>AFEDRDPTQFEERHLKFLRQLGKGNFGSVEMCRYDPLQDNTGEVVAVKKLQHSTEEHLRDFEREIEILKSLQHDNIVKYKGVCYSAGRRNLKLIMEFLPYGSLREYLQKHKERIDHIKLLQYTSQICKGMEYLGTKRYIHRDLATRNILVENENRVKIGDFGLTKVLPQDKEYYKVKEPGESPIFWYAPESLTESKFSVASDVWSFGVVLYELFTYIEKSKSPPAEFMRMIGNDKQGQMIVFHLIELLKNNGRLPRPDGCPDEIYMIM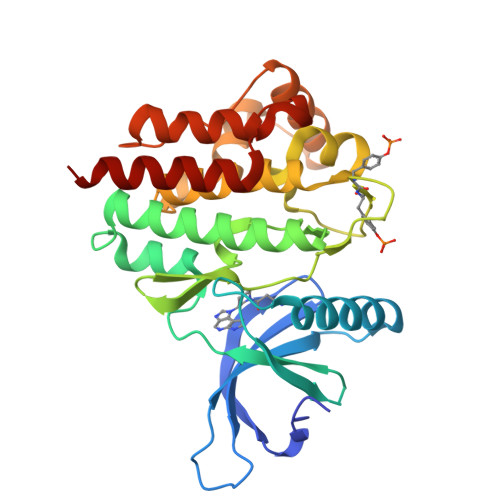TECWNNNVNQRPSFRDLALRVDQIRDNMAG[2x]>[3x]SKKWFSEFSIMWPGQAFSLKIKKILYETKSKYQN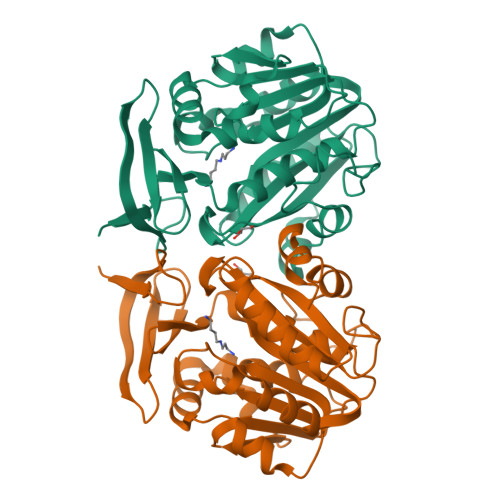VLVFESTTYGKVLVLDGVIQLTEKDEFAYHEMMTHVPMTVSKEPKNVLVVGGGDGGIIRELCKYKSVENIDICEIDETVIEVSKIYFKNISCGYEDKRVNVFIEDASKFLENVTNTYDVIIVDSSDPIGPAETLFNQNFYEKIYNALKPNGYCVAQCESLWIHVGTIKNMIGYAKKLFKKVEYANISIPTYPCGCIGILCCSKTDTGLTKPNKKLESKEFADLKYYNYENHSAAFKLPAFLLKEIENI> MKEFYLTVEQIGDSIFERYIDSNGRERTREVEYKPSLFAHCPESQAT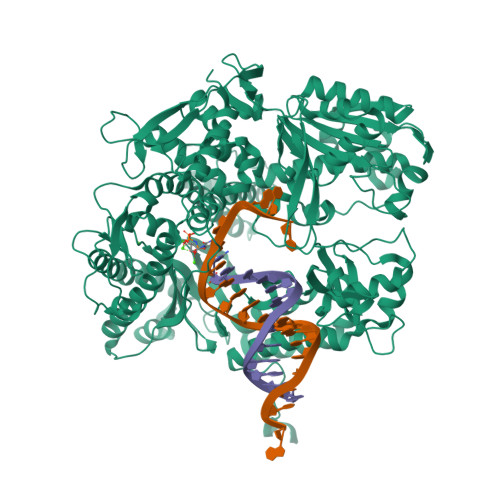KYFDIYGKPCTRKLFANMRDASQWIKRMEDIGLEALGMDDFKLAYLSDTYNYEIKYDHTKIRVANFDIEVTSPDGFPEPSQAKHPIDAITHYDSIDDRFYVFDLLNSPYGNVEEWSIEIAAKLQEQGGDEVPSEIIDKIIYMPFDNEKELLMEYLNFWQQKTPVILTGWNVESFAIPYVYNRIKNIFGESTAKRLSPHRKTRVKVIENMYGSREIITLFGISVLDYIDLYKKFSFTNQPSYSLDYISEFELNVGKLKYDGPISKLRESNHQRYISYNIIAVYRVLQIDAKRQFINLSLDMGYYAKIQIQSVFSPIKTWDAIIFNSLKEQNKVIPQGRSHPVQPYPGAFVKEPIPNRYKYVMSFDLTSLYPSIIRQVNISPETIAGTFKVAPLHDYINAVAERPSDVYSCSPNGMMYYKDRDGVVPTEITKVFNQRKEHKGYMLAAQRNGEIIKEALHNPNLSVDEPLDVDYRFDFSDEIKEKIKKLSAKSLNEMLFRAQRTEVAGMTAQINRKLLINSLYGALGNVWFRYYDLRNATAITTFGQMALQWIERKVNEYLNEVCGTEGEAFVLYGDTDSIYVSADKIIDKVGESKFRDTNHWVDFLDKFARERMEPAIDRGFREMCEYMNNKQHLMFMDREAIAGPPLGSKGIGGFWTGKKRYALNVWDMEGTRYAEPKLKIMGLETQKSSTPKAVQKALKECIRRMLQEGEESLQEYFKEFEKEFRQLNYISIASVSSANNIAKYDVGGFPGPKCPFHIRGILTYNRAIKGNIDAPQVVEGEKVYVLPLREGNPFGDKCIAWPSGTEITDLIKDDVLHWMDYTVLLEKTFIKPLEGFTSAAKLDYEKKASLFDMF>GPHMKHPLMNVWTLWYLENDRSKSWEDMQNEITSFDTVEDFWSLYNHIKPPSEIKLGSDYSLFKKNIRPMWEDAANKQGGRWVITLNKSSKTDLDNLWLDVLLCLIGEAFDHSDQICGAVINIRGKSNKISIWTADGNNEEAALEIGHKLRD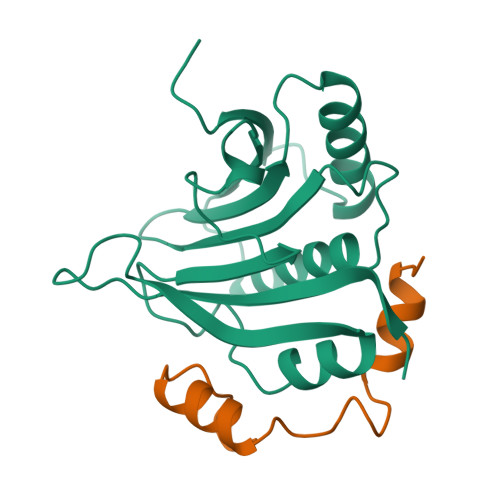ALRLGRNNSLQYQLHKDTMVKQGSNVKSIYTL[3x];>GPHMLERYSKVDLLALRYSPLSQTPPGIELEGRLRRMNIWRTGS[3x]4-[(3S)-3-({[(E)-2-(5-chlorothiophen-2-yl)ethenyl]sulfonyl}amino)-2-oxopyrrolidin-1-yl]-3-fluoro-N,N-dimethylbenzamide | C19 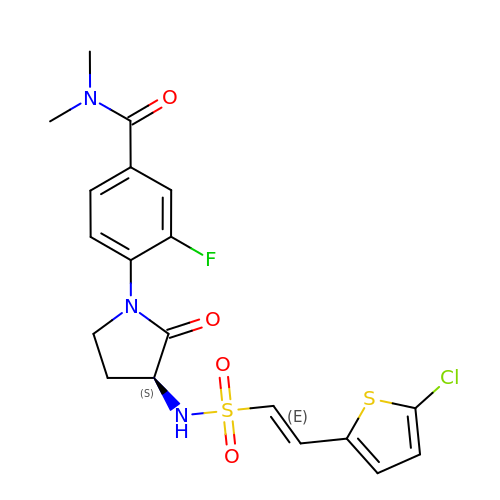H19 Cl F N3 O4 S2 | YVFKLOGRKAMHKF-HQPKTYMTSA-N> MASVHGTTYELLRRQGIDTVFGNPGSNQLPFLKDFPEDFRYILALQEACVVGIADGYAQASRKPAFINLHSAAGTGNAMGALSNAWNSHSPLIVTAGQQTRAMIGVEALLTNVDAANLPRPLVKWSYEPASAAEVPHAMSRAIHMASMAPQGPVYLSVPYDDWDKDADPQSHHLFDRHVSSSVRLNDQDLDILVKALNSA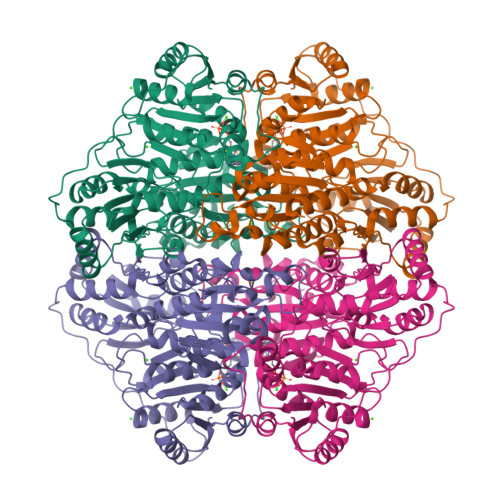SNPAIVLGPDVDAANANADCVMLAERLKAPVWVAPSAPRCPFPTRHPCFRGLMPAGIAAISQLLEGHDVVLVIGAPVFRYHQYDPGQYLKPGTRLISVTCDPLEAARAPMGDAIVADIGAMASALANLVEESSRQLPTAAPEPAKVDQDAGRLHPETVFDTLNDMAPENAIYLNESTSTTAQMWQRLNMRNPGSYYFCAAGGLGFALPAAIGVQLAEPERQVIAVIGDGSANYSISALWTAAQYNIPTIFVIMNNGTYGALRWFAGVLEAENVPGLDVPGIDFRALAKGYGVQALKADNLEQLKGSLQEALSAKGPVLIEVSTVSPVK> MKIMKEFKEQFGYQLSNFDDMDIKGYANLYQKDIGKDVSMIEQGLKQLSITETEVLLPEQINKKLLGVLNMNEVNQSSNTWVGTLTKQLVSSENNFNIQELPTARKEVFKELLVNRELPQTLRDVITITDDEHVESIPALSYIKDKLATNGIELSLNGSSKYFDRREGHIYTEVADSVVHGSDRTLDDLLKEIFINECVSYETTLLLDKNNASGLIDKDNQDLSLYNQGIKEVSNTSMYDGIKQAMKDIPQTFRRKVSVVMNTEHHDKLIKELAQMGLGTLAGDLTKLFNVSHVVVTDDAQDIFVGDFGHAIYAKYEPIMYNKKKQALKGVYQFALNYVFDI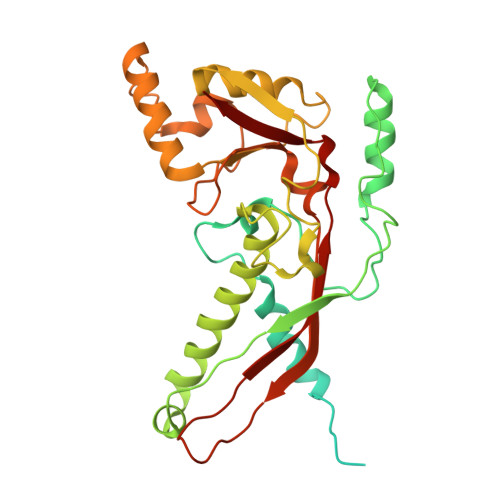KIVPELLRIVKVK> MGSDKIHHHHHHENLYFQGMRNMQEKGVSEKEILEELKKYRSLDLKYEDGNIFGSMCSNVLPITRKIVDIFLETNLGDPGLFKGTKLLEEKAVALLGSLLNNKDAYGHIVSGGTEANLMALRCIKNIWREK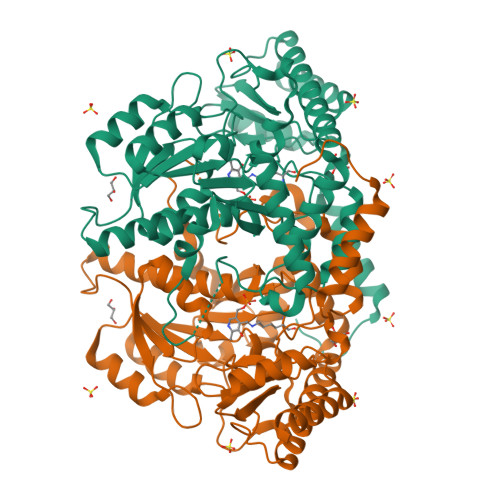RRKGLSKNEHPKIIVPITAHFSFEKGREMMDLEYIYAPIKEDYTIDEKFVKDAVEDYDVDGIIGIAGTTELGTIDNIEELSKIAKENNIYIHVDAAFGGLVIPFLDDKYKKKGVNYKFDFSLGVDSITIDPHKMGHCPIPSGGILFKDIGYKRYLDVDAPYLTETRQATILGTRVGFGGACTYAVLRYLGREGQRKIVNECMENTLYLYKKLKENNFKPVIEPILNIVAIEDEDYKEVCKKLRDRGIYVSVCNCVKALAIVVMPHIKREHIDNFIEILNSIKRD(1R,4R,5R)-1,4,5-trihydroxy-3-[3-(phenylcarbonyl)phenyl]cyclohex-2-ene-1-carboxylic acid | C20 H18 O6 | 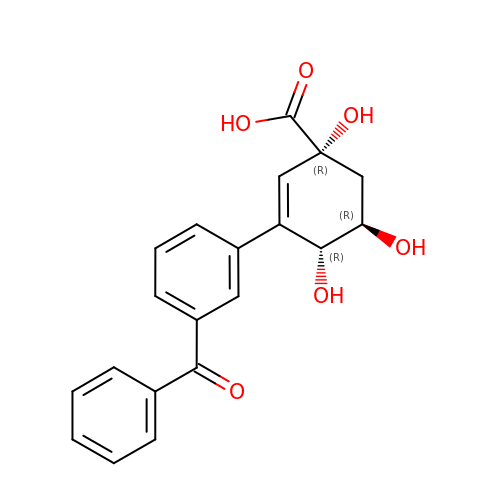XHOCFTKQBAZROZ-POAQFYNOSA-N> F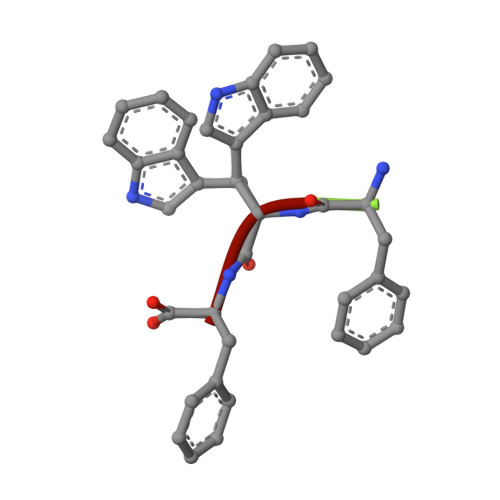WF> PRKIILDCDPGIDDAVAILL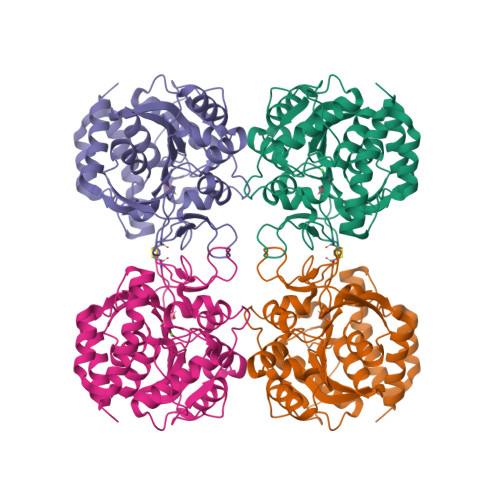AYGNPEIELLAITTVVGNQTLEKVTRNAQLVADVAGIVGVPIAAGCCKPLVRKVRTAPQIHGETGLGTVSYPSEFKTKLDKRHAVHLIIELIMSHEPKSITLVPTGGLTNIAMAARLEPRIVERVKEVVLMGGSCCIGNASPVAEFNIFVDPEAAHIVFNESWDVTMVGLDLTSQALATPEVLQRVKEVRTKPADFILKILEFYTKVYETQRNTYAKVHDPCAVAYVIDPTVMTTNRVPVNIELNGELTAGMTVTDFRYPRPEQCHTQVASKLDFSKYWDLVIDALQRIGDP SARS-CoV-2 is a positive-strand RNA virus. Its replication is mediated by a multisubunit replication-and-transcription complex of viral nonstructural proteins (nsps). The core component of this complex is the catalytic subunit (nsp12) of an RNA-dependent RNA polymerase (RdRp). By itself, nsp12 has little activity and its functions require accessory factors, including nsp7 and nsp8 (14, 15), that increase RdRp template binding and processivity.

For the apo nsp12-nsp7-nsp8 complex, we vitrified the sample in the presence of the detergent DDM. The structure of the apo RdRp complex contains one nsp12, one nsp7, and two nsp8 proteins, with an overall arrangement resembling those seen in SARS-CoV and the recently solved structure of SARS-CoV-2 (15, 23). Our structure, which differs from the SARS-CoV RdRp structure but is similar to the recent SARS-CoV-2 RdRp structure, reveals that nsp12 also contains an N-terminal β hairpin (residues 31 to 50) and an extended nidovirus RdRp-associated nucleotidyl-transferase domain (NiRAN; residues 115 to 250) with seven helices and three β strands. After the NiRAN domain is an interface domain (residues 251 to 365), composed of three helices and five β strands, that is connected to the RdRp domain (residues 366 to 920). The nsp12 RdRp domain displays the canonical cupped right-handed configuration, with the finger subdomain (residues 397 to 581 and 621 to 679) forming a closed circle with the thumb subdomain (residues 819 to 920). The closed conformation is stabilized by the binding of nsp7 and nsp8, with one nsp8 molecule sitting atop the finger subdomain and interacting with the interface domain. The closed conformation of nsp12 is further stabilized by the nsp7-nsp8 heterodimer, which is packed against the thumb-finger interface. In addition, we were able to assign two zinc ions in the conserved metal binding motifs composed of H295-C301-C306-C310 and C487-H642-C645-C646, which are also observed in the SARS-CoV RdRp structure. These zinc ions likely function as conserved structural components in maintaining the integrity of the RdRp architecture. Outside of these changes, the apo nsp12 and the RNA complex nsp12 are very similar, with a root mean square deviation of 0.52 Å for all Cα atoms across the whole protein.

> MSADAQSFLNRVCGVSAARLTPCGTGTSTDVVYRAFDIYNDKVAGFAKFLKTNCCRFQEKDEDDNLIDSYFVVKRHTFSNYQHEETIYNLLKDCPAVAKHDFFKFRIDGDMVPHISRQRLTKYTMADLVYALRHFDEGNCDTLKEILVTYNCCDDDYFNKKDWYDFVENPDILRVYANLGERVRQALLKTVQFCDAMRNAGIVGVLTLDNQDLNGNWYDFGDFIQTTPGSGVPVVDSYYSLLMPILTLTRALTAESHVDTDLTKPYIKWDLLKYDFTEERLKLFDRYFKYWDQTYHPNCVNCLDDRCILHCANFNVLFSTVFPPTSFGPLVRKIFVDGVPFVVSTGYHFRELGVVHNQDVNLHSSRLSFKELLVYAADPAMHAASGNLLLDKRTTCFSVAALTNNVAFQTVKPGNFNKDFYDFAVSKGFFKEGSSVELKHFFFAQDGNAAISDYDYYRYNLPTMCDIRQLLFVVEVVDKYFDCYDGGCINANQVIVNNLDKSAGFPFNKWGKARLYYDSMSYEDQDALFAYTKRNVIPTITQMNLKYAISAKNRARTVAGVSICSTMTNRQFHQKLLKSIAATRGATVVIGTSKFYGGWHNMLKTVYSDVENPHLMGWDYPKCDRAMPNMLRIMASLVLARKHTTCCSLSHRFYRLANECAQVLSEMVMCGGSLYVKPGGTSSGDATTAYANSVFNICQAVTANVNALLSTDGNKIADKYVRNLQHRLYECLYRNRDVDTDFVNEFYAYLRKHFSMMILSDDAVVCFNSTYASQGLVASIKNFKSVLYYQNNVFMSEAKCWTETDLTKGPHEFCSQHTMLVKQGDDYVYLPYPDPSRILGAGCFVDDIVKTDGTLMIERFVSLAIDAYPLTKHPNQEYADVFHLYLQYIRKLHDELTGHMLDMYSVMLTNDNTSRYWEPEFYEAMYTPHTVLQGGSENLYFQGHHHHHHHH;>MAIASEFSSLPSYAAFATAQEAYEQAVANGDSEVVLKKLKKSLNVAKSEFDRDAAMQRKLEKMADQAMTQMYKQARSEDKRAKVTSAMQTMLFTMLRKLDNDALNNIINNARDGCVPLNIIPLTTAAKLMVVIPDYNTYKNTCDGTTFTYASALWEIQQVVDADSKIVQLSEISMDNSPNLAWPLIVTALRANSAVKLQHHHHHHHH[2x];> MSKMSDVKCTSVVLLSVLQQLRVESSSKLWAQCVQLHNDILLAKDTTEAFEKMVSLLSVLLSMQGAVDINKLCEEMLDNRATLQHHHHHHHH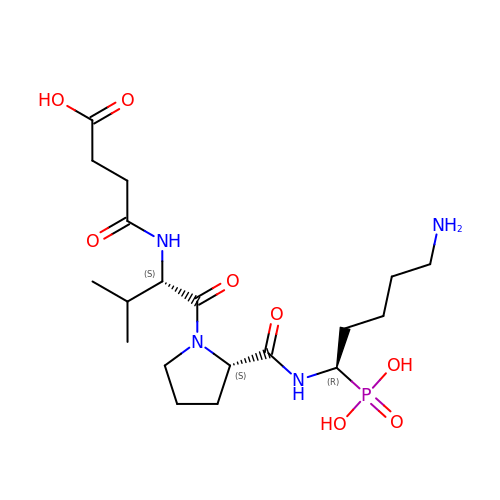N-(3-carboxypropanoyl)-L-valyl-N-[(1R)-5-amino-1-phosphonopentyl]-L-prolinamide | C19 H35 N4 O8 P | POVVCGMAFFRCCC-LXZKKBNFSA-N>MMDTQRPLDALGKSI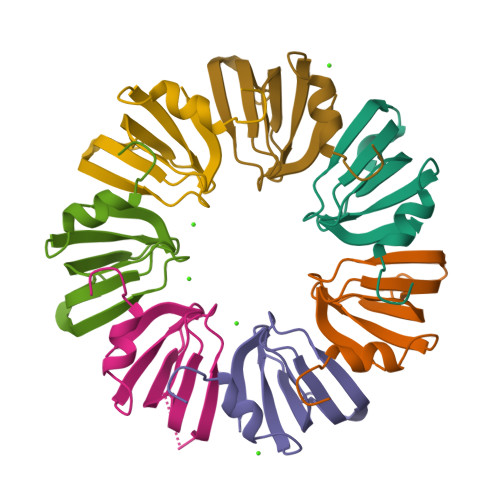NTNVTVYLKDGKLVKGRLKAYDLHMNVALENAKIESDEEKEFPMLVVRGDNVLYVSL[14x]>[12x]MEALGMIETRGLVALIEASDAMVKAARVKLVGVKQIGGGLC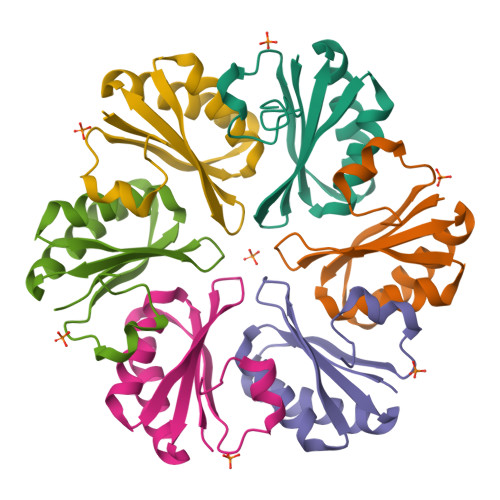TAMVRGDVAACKAATDAGAAAAQRIGELVSVHVIPRPHGDLEEVFPIGLKGDSSNLHHHHHH>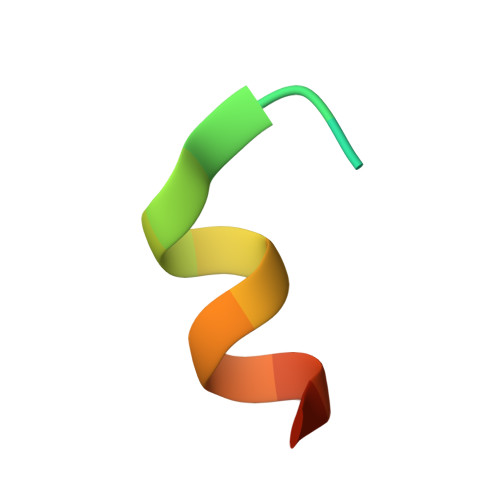 MSDQFNSREARRKANSK> MSQGDSNPAAIPHAAEDIQGDDRWMSQH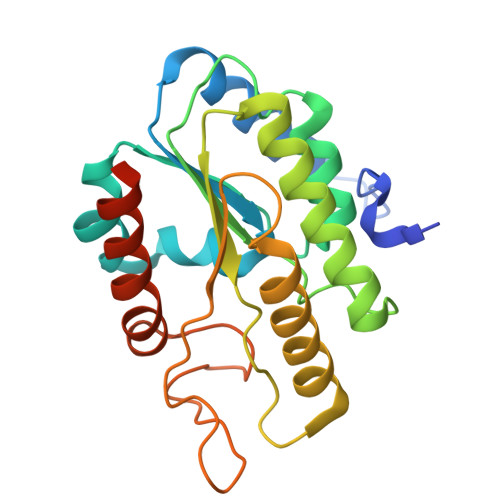NRFVLDCKDKEPDVLFVGDSMVQLMQQYEIWRELFSPLHALNFGIGGDTTRHVLWRLKNGELENIKPKVIVVWVGTNNHENTAEEVAGGIEAIVQLINTRQPQAKIIVLGLLPRGEKPNPLRQKNAKVNQLLKVSLPKLANVQLLDTDGGFVHSDGAISCHDMFDFLHLTGGGYAKICKPLHELIMQLLEETPEEKQTTIA> MSIQHFRVALIPFFAAFCLPVFAHPETLVKVKDAEDQLGARVGYIELDLNSGKILESFRPEERFPMMSTFKVLLCGAVLSRIDAGQEQLGRRIHYSQNDLVEYSPVTEKHLTDGMTVRELCSAAITMSDNTAANLLLTTIGGPKELTAFLHNMGDHVTRLDRWEPELNEAIPNDERDTTMPVAMATTLRKLLTGELLTLASR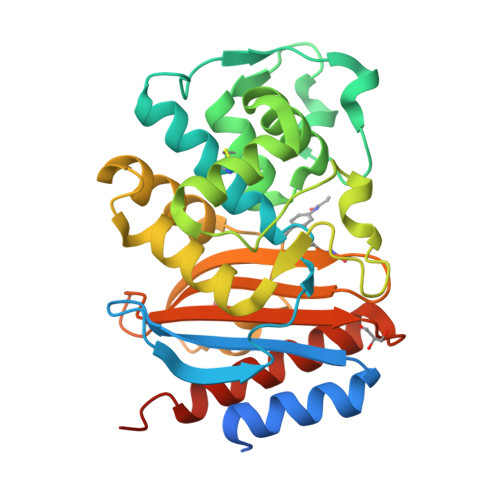QQLIDWMEADKXAGPLLRSALPAGWFIADKSGAGERGSRGIIAALGPDGKPSRIVVIYTTGSQATMDERNRQIAEIGASLIKHWAAALEHHHHHH> MSKKYTQQQYEKYLAQPANNTFGLSPQQVADWFMGQAGARPVINSYGVNASNLVSTYIPKMQEYGVSYTLFLMYTVFEGGGAGNWINHYMYDTGSNGLECLEHDLQYIHGVWETYFPPALSAPECYPATEDNAGALDRFYQSLPGRTWGDVMIPSTMAGNAWVWAYNYCVNNQGAAPLVYFGNPYDSQIDSLLAMGADPFTGGSITGDGKNPSVGTGNATVSASSEANREKLKKALTDLFNNNLEHLSGEFYGNQVLNAMKYGTILKCDLTDDGLNAILQLIADVNLQTNPNPDKPTVQSPGQNDLGSGSDRVAANLANAQAQVGKYIGDGQCYAWVGWWSARVCGYSISYSTGDPMLPLIGDGMNAHSIHLGWDWSIANTGIVNYPVGTVGRKEDLRVGAIWCATAFSGAPFYTGQYGHTGIIESWS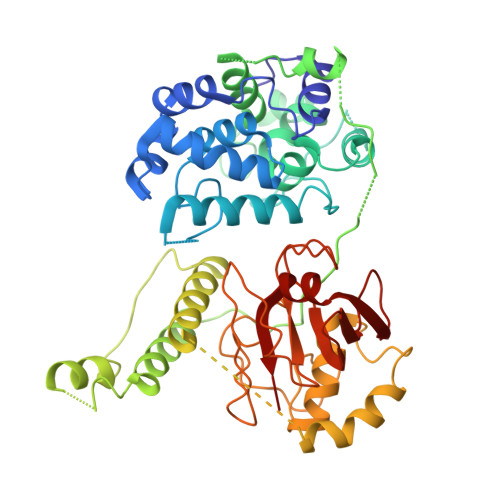DTTVTVLEQNILGSPVIRSTYDLNTFLSTLTGLITFK> MGSSHHHHHHSQDPMSLIKKKNKDIRIIPLGGVGEIAKNMYIVEVDDEMFMLDAGLMFPEDEMLGVDIVIPDIQYVIENKERLKGIFLTHGHEHAIGAVSYVLEQIDAPVYGSKLTIALVKEAMKARNIKKKVRYYTVNHDSIMRFKNVNVSFFNTTASIPDSLGVCIHTSYGSIVYTGEFKFDQSLHGHYAPDLKRMAEIGDEGVFALISDSTEAEKPGYNTPENIIEHHMYDAFAKVKGRLIVSCYASNFVRIQQVLNIASQLNRKVSFLGRSLESSFNIARKMGYFDIPKDLLIPINEVENYPKNEVIIIATGMQGEPVEALS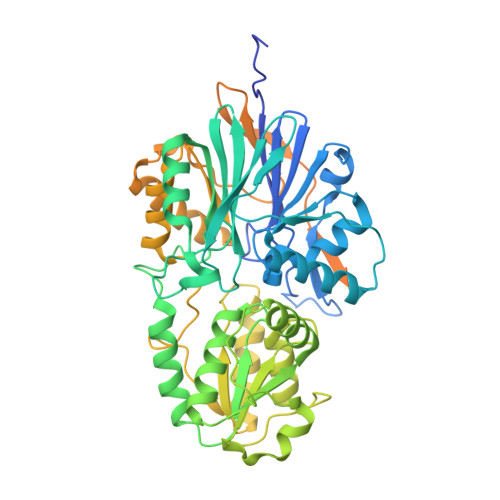QMARKKHKIMNIEEGDSIFLAITASANMEVIIADTLNELVRAGAHIIPNNKKIHASSHGCMEELKMMLNIMKPEYFVPVQGEFKMQIAHAKLAAETGVAPEKIFLVEKGDVISYNGKDMILNEKVQSGNILIDGIGVGDVGNIVLRDRHLLAEDGIFIAVVTLDPKNRRIAAGPEIQSRGFVYVRESEELLKEAEEKVRKIVEEGLQEKRIEWSEIKQNMRDQISKLLFESTKRRPMIIPVISEI> GIPPKIEA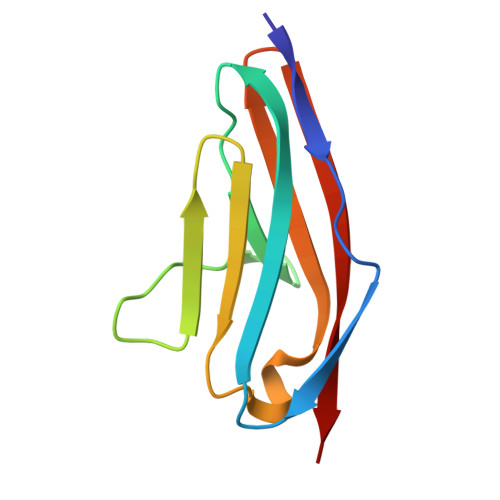LPSDISIDEGKVLTVACAFTGEPTPEVTWSCGGRKIHSQEQGRFHIENTDDLTTLIIMDVQKQDGGLYTLSLGNEFGSDSATVNIHIRS>MIKQRTLKNIIRATGVGLHSGEKVYLTLKPAPVDTGIVFCRTDLDPVVEIPARAENVGETTMSTTLVKGDVKVDTVEHLLSAMAGLGIDNAYVELSASEVPIMDGSAGPFVFLIQSAGLQEQEAAKKFIRIKREVSVEEGD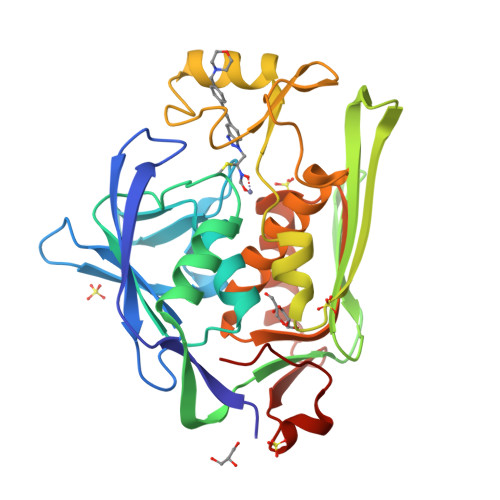KRAVFVPFDGFKVSFEIDFDHPVFRGRTQQASVDFSSTSFVKEVSRARTFGFMRDIEYLRSQNLALGGSVENAIVVDENRVLNEDGLRYEDEFVKHKILDAIGDLYLLGNSLIGEFRGFKSGHALNNQLLRTLIADKDAWEVVTFEDARTAPISYMRPAAAV[2x]>GDYLHLPSEVSRFFRPQETNDDHGEDSVGTRWAVLIAGSKGYANYRHQAGVCHAYQILKRGGLKDENIVVFMYDDIAYNESNPRPGVIINSPHGSDVYAGVPKDYTGEEVNAKNFLAAILGNKSAITGGSGKVVDSGPNDHIFIYYTDHGAAGVIGMPSKPYLYADELNDALKKKHASGTYKSLVFYLEACESGSMFEGILPEDLNIYALTSTNTTESSWCYYCPAQENPPPPEYNVCLGDLFSVAWLEDSDVQNSWYETLNQQYHHVDKRISHASHATQYGN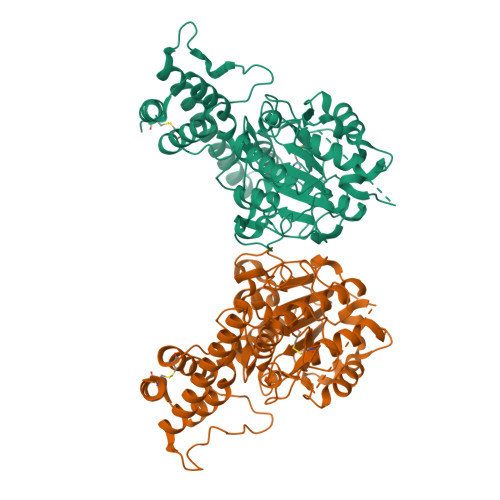LKLGEEGLFVYMGSNPANDNYTSLDGNALTPSSIVVNQRDADLLHLWEKFRKAPEGSARKEEAQTQIFKAMSHRVHIDSSIKLIGKLLFGIEKCTEILNAVRPAGQPLVDDWACLRSLVGTFETHCGSLSEYGMRHTRTIANICNAGISEEQMAEAASQACASIP[2x]>MSRGDKMLKFEIKARDGAGRIGKLEVNGKKIETPAIMPVVNPKQMVVEPKELEKMGFEIIITNSYIIYKDEELRRKALELGIHRMLDYNGIIEVDSGSFQLMKYGSIEVSNREIIEFQHRIGVDIGTFLDIPTPPDAPREQAVKELEITLSRAREAEEIKEIPMNATIQGSTYTDLRRYAARRLSSMNFEIHPIGGVVPLLESYRFRDVVDIVISSKMALRPDRPVHLFGAGHPIVFALAVAMGVDLFDSASYALYAKDDRYMTPEGTKRLDELDYFPCSCPVCSKYTPQELREMPKEERTRLLALHNLWVIKEEIKRVKQAIKEGELWRLVDERARSHPKLYSAYKRLLEHYTFLEEFEPITKKSALFKISNESLRWPVVRRAKERAKSINERFGELVEHPIFGRVSRYLSLTYPFAQSEAEDDFKIEKPTKEDAIKYVMAIAEYQFGEGASRAFDDAKVELSKTGMPRQVKVNGKRLATVRADDGLLTLGIEGAKRLHRVLPYPRMRVVVNKEAEPFARKGKDVFAKFVIFADPGIRPYDEVLVVNENDELLATGQALLS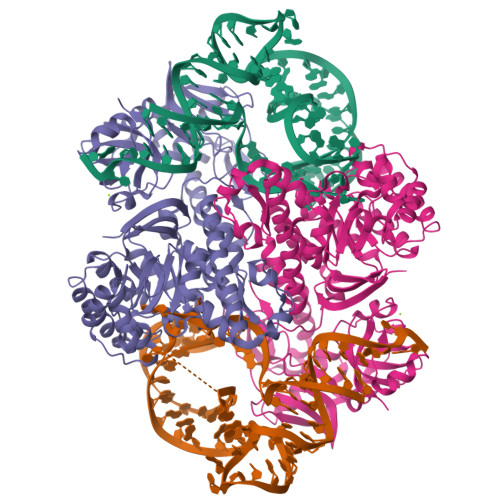GREMIVFQYGRAVKVRKGVE[2x]>CSLAPDYQRPAMPVPQQFSLSQNGLVNAADNYQNAGWRTFFVDNQVKTLISEALVNNRDLRMATLKVQEARAQYRLTDADRYPQLNGEGSGSWSGNLKGNTATTREFSTGLNASFDLDFFGRLKNMSEAERQNYLATEEAQRAVHILLVSNVAQSYFNQQLAYAQLQIAEETLRNYQQSYAFVEKQLLTGSSNVLALEQARGVIESTRSDIAKRQGELAQANNALQLLLGSYGKLPQAQTVNSDSLQSVKLPAGLSSQILLQRPDIMEAEHALMAANANIGAAR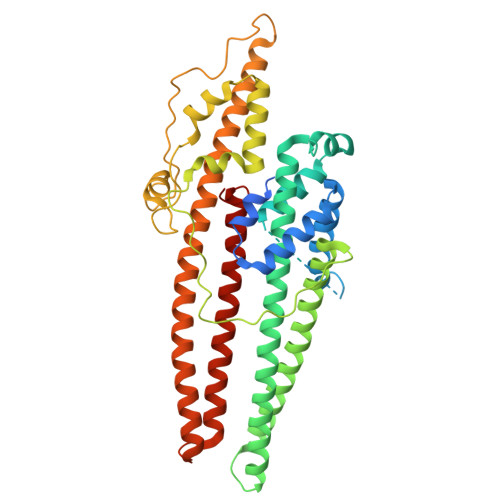AAFFPSISLTSGISTASSDLSSLFNASSGMWNFIPKIEIPIFNAGRNQANLDIAEIRQQQSVVNYEQKIQNAFKEVADALALRQSLNDQISAQQRYLASLQITLQRARALYQHGAVSYLEVLDAERSLFATRQTLLDLNYARQVNEISLYTALGGGHHHHHH[2x]> MEIKRFGRIREVIPLPPLTEIQVESYKKALQADVPPEKRENVGIQAAFKETFPIEEGDKGKGGLVLDFLEYRIGDPPFSQDECREKDLTYQAPLYARLQLIHKDTGLIKEDEVFLGHLPLMTEDGSFIINGADRVIVSQIHRSPGVYFTPDPARPGRYIASIIPLPKRGPWIDLEVEASGVVTMKVNKRKFPLVLLLRVLGYDQETLVRELSAYGDLVQGLLDEAVLAMRPEEAMVRLFTLLRPGDPPKKDKALAYLFGLLADPKRYDLGEAGRYKAEEKLGVGLSGRTLVRFEDGEFKDEVFLPTLRYLFALTAGVPGHEVDDIDHLGNRRIRTVGELMADQFRVGLARLARGVRERMVMGSPDTLTPAKLVNSRPLEAALREFFSRSQLSQFKDETNPLSSLRHKRRISALGPGGLTRERAGFDVRDVHRTHYGRICPVETPEGANIGLITSLAAYARVDALGFIRTPYRRVKNGVVTEEVVYMTASEEDRYTIAQANTPLEGDRIATDRVVARRRGEPVIVAPEEVEFMDVSPKQVFSLNTNLIPFLEHDDANRALMGSNMQTQAVPLIRAQAPVVMTGLEERVVRDSLAALYAEEDGEVVKVDGTRIAVRYEDGRLVHPLRRYARSNQGTAFDQRPRVRVGQRVKKGDLLADGPASEEGFLALGQNVLVAIMPFDGYNFEDAI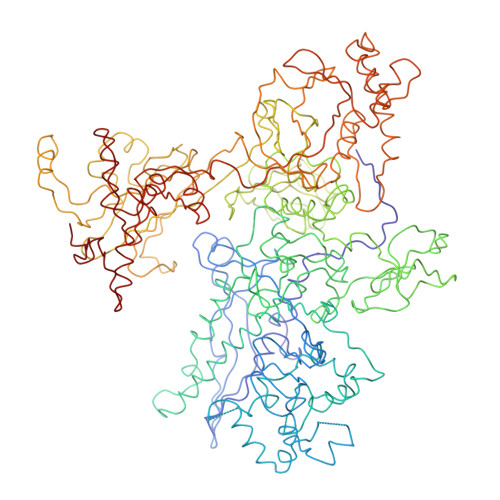VISEELLKRDFYTSIHIERYEIEARDTKLGPERITRDIPHLSEAALRDLDEEGIVRIGAEVKPGDILVGRTSFKGEQEPSPEERLLRSIFGEKARDVKDTSLRVPPGEGGIVVGRLRLRRGDPGVELKPGVREVVRVFVAQKRKLQVGDKLANRHGNKGVVAKILPVEDMPHLPDGTPVDVILNPLGVPSRMNLGQILETHLGLAGYFLGQRYISPVFDGATEPEIKELLAEAFNLYFGKRQGEGFGVDKREKEVLARAEKLGLVSPGKSPEEQLKELFDLGKVVLYDGRTGEPFEGPIVVGQMFIMKLYHMVEDKMHARSTGPYSLITQQPLGGKAQFGGQRFGEMEVWALEAYGAAHTLQEMLTIKSDDIEGRNAAYQAIIKGEDVPEPSVPESFRVLVKELQALALDVQTLDEKDNPVDIFEGLASKR>MLQNSFKLAQSLRNGFYRNAWRAFSSHGPRQPLVSPERRLEKAHPTFTERSQLKYARRLVVKLGSAVITREDNHGLALGRLASIVEQVAECHLEGREVMMVTSGAVAFGKQKLAQELLMSLSMRETLNPKDSKEFDGATLEPRAAAAVGQSGLMSLYDAMFAQYGVKIAQVLVTKPDFYNEETRNNLFCTLSELISLNIVPIINTNDAVSPPMFIRDDEPAGGARRGIPIKDNDSLSAMLAAEVQADLLILMSDVDGIYNKPPWEDGAKLMHTYTSDDSNSIEFGKKSKVGTGGMDSKVKAATWALDRGVSVVICNGMQEKAIKTIIGGRKVGTFFTEATESANAVPVEVMAENARTGSRQMQALTPAQRASAVNTLADLLVSREKFILDANAKDLAEAQKSGLAKPLLSRLSLNPAKLKNLSVGLKQIAEDSHKNVGRVLRRTRLADQLELKQVTVPIGVLLVIFESRPDSLPQVAALAMASANGLLLKGGKEAAHSNKALMELVKEALATVGAEHAVSLVSTREEISDLLSMENHIDLIIPRGSSDLVRSIQQQSLHIPVLGHAEGVCHVYIDRDADLEKALRIARDAKCDYPAACNAMETLLIHEDLMSGAIFGDVCNMLKREGVKIYAGPRLNQQLTFGPPAAKSLKHEYGALECCIEVVPSLDEAINHIHTYGSSHTDVIVTENDAAARQFLGSVDSACVFHNASSRFADGFRFGLGAEVGISTARIHARGPVGVEGLLTTKWILEGQDHAAADFAEGGGRTWLHE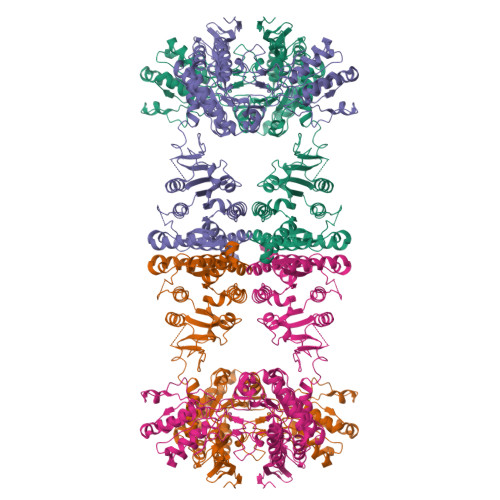TLPLD[4x]>MPAKTLESKDYCGESFVSEDRSGQSLESIRFEDCTFRQCNFTEAELNRCKFRECEFVDCNLSLISIPQTSFMEVRFVDCKMLGVNWTSAQWPSVKMEGALSFERCILNDSLFYGLYLAGVKMVECRIHDANFTEADCEDADFTQSDLKGSTF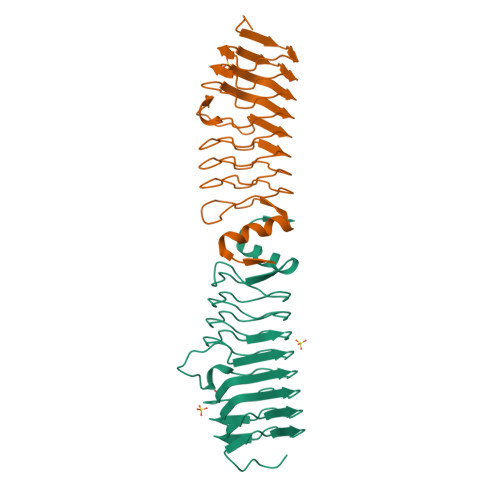HNTKLTGASFIDAVNYHIDIFHNDIKRARFSLPEAASLLNSLDIELSD[2x]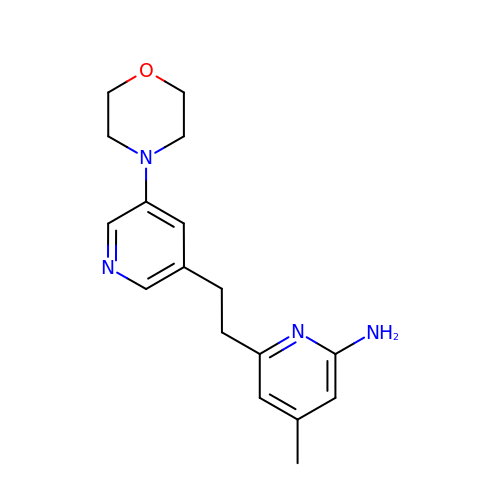4-methyl-6-[2-(5-morpholin-4-ylpyridin-3-yl)ethyl]pyridin-2-amine | C17 H22 N4 O | ILLMLHPSAJJCTB-UHFFFAOYSA-N>[4x]MASMTGGQQMGRGSAGVLPAHGTQHGIRLPLRSGLGGAPLGLRLPRETDEEPEEPGRRGSFVEMVDNLRGKSGQGYYVEMTVGSPPQTLNILVDTGSSNFAVGAAPHPFLHRYYQRQLSSTYRDLRKGVYVPYTQGKWEGELGTDLVSIPHGPNVTVRANIAAITESDKFFINGSNWEGILGLAYAEIARPDDSLEPFFDSLVKQTHVPN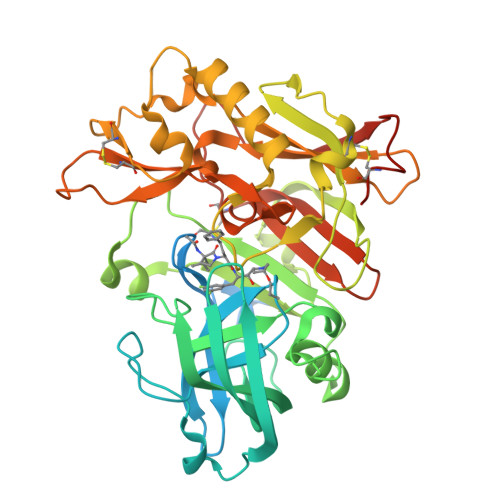LFSLQLCGAGFPLNQSEVLASVGGSMIIGGIDHSLYTGSLWYTPIRREWYYEVIIVRVEINGQDLKMDCKEYNYDKSIVDSGTTNLRLPKKVFEAAVKSIKAASSTEKFPDGFWLGEQLVCWQAGTTPWNIFPVISLYLMGEVTNQSFRITILPQQYLRPVEDVATSQDDCYKFAISQSSTGTVMGAVIMEGFYVVFDRARKRIGFAVSACHVHDEFRTAAVEGPFVTLDMEDCGYNIPQTDEST>QYEAFKDMLYSAQDQAPSVEVTDEDTVKRYFAKFEEKFFQTCEKELAKINTFYSEKLAEAQRRFATLQNELQSSLDAQKESTGVTTLRQRRKPVFHLSHEERVQHRNIKDLKLAFSEFYLSLILLQNYQNLNFTGFRKILKKHDKILETSRGADWRVAHVEVAPFYTCKKINQLISETEAVVTNELEDGDRQKAMKRLRVPPLGAAQPAPAWTTFRVGLFCGIFIVLNITLVLAAVFKLETDRSIWPLIRIYRGGFLLIEFLFLLGINTYGWRQAGVNHVLIFELNPRSNLSHQHLFEIAGFLGILWCLSLLACFFAPISVIPTYVYPLALYGFMVFFLINPTKTFYYKSRFWLLKLLFRVFTAPFHKVGFA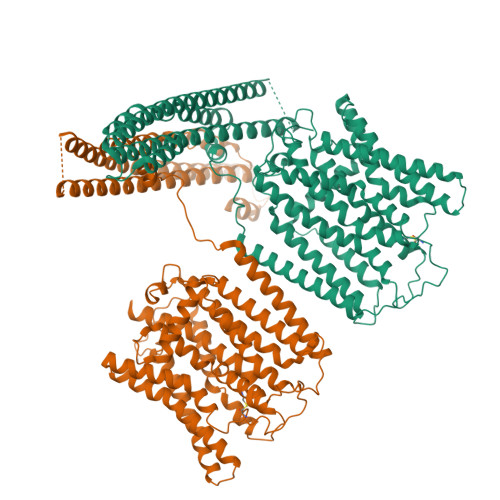DFWLADQLNSLSVILMDLEYMICFYSLELKWDESKGLLPNNSEESGICHKYTYGVRAIVQCIPAWLRFIQCLRRYRDTKRAFPHLVNAGKYSTTFFMVTFAALYSTHKERGHSDTMVFFYLWIVFYIISSCYTLIWDLKMDWGLFDKNAGENTFLREEIVYPQKAYYYCAIIEDVILRFAWTIQISITSTTLLPHSGDIIATVFAPLEVFRRFVWNFFRLENEHLNNC[2x]> PLQPSFTPSVAFPAHKPVPLNSPLSPSVHAAPQVRRPGSVVRMNEVIRHWWSVPAVGFNSVLEVPIYRFEVFQRRAEEAGEGEASIAEEGDHPEEEEGCVVLPNDIFGLPLRPDILYRCYWFYRRAIAGWTERMQLFKWEWPGSKRKLRTQQRSGRARIGWRKAPGKYVGVKAHPLRPH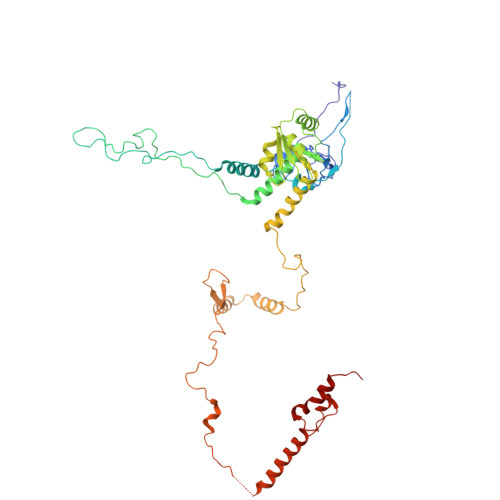DQRIKINKRLLWQGLKIMLSAKFAQGQITVVDHFNLQSHKTKHCVRHLRRLLGRKCPSALLVHEGTTDVNDNFRYATAHILAVRRENVEGINVYNLLKYRQLVITEKALLKLIYNIQTYPEKRGWLPKYATPDGKPAPAPEKVEGWDREWRQMKERERNAKFSKALLRERILKWKWSDETKGAIKVPRVDPFKGFRLARFSLHEPTMPWEKFEENYVDTDPLEDEEDGDMFDEAQALGEETQRLERLDHEELSDAAAYDDMSLTDMPLTERMHRPKRLENFKMEP> VPDEWEVAREKITMSRELGQGSFGMVYEGVAKGVVKDEPETRVAIKTVNEAASMRERIEFLNEASVMKEFNCHHVVRLLGVVSQGQPTLVIMELMTRGDLKSYLRSLRPEMENNPVLAPPSLSKMIQMAGEIADGMAYLNANKFVHRDLAARNCMVAEDFTVKIGDFGMTRDIYETDYYRKGGKGLLPVRWMSPESLKDGVFTTYSDVWSFGVVLWE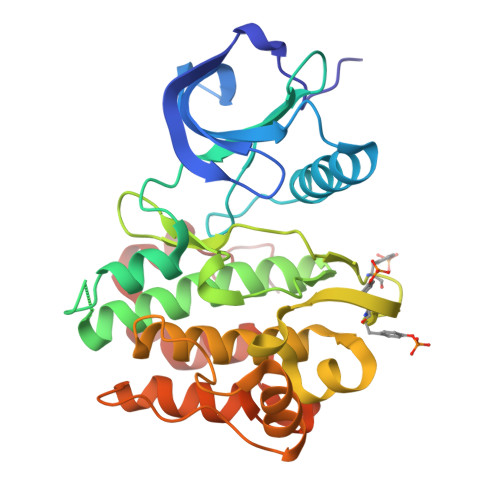IATLAEQPYQGLSNEQVLRFVMEGGLLDKPDNCPDMLLELMRMCWQYNPKMRPSFLEIISSIKEEMEPGFREVSFYYSEENK> GUGCGACAAGAAGUUCAGGAAGGGAUUGAGGUGAAAGUCCUCCUCCCGAAUCGUUCAUGGGAGAGUCUAUCCAGACUUGCGUAGCGAGUAAUCGCUAGGUGAGAAGCUCUGGAGACAAUGUACCUGCCCUUCAAUUGGAGGUGCCAGGGCUAGGCUUUGUUCCUAUGGCUAGCGAAAGCGAAUACAGGUUAUUAGGCGUCGUGAAAACAAAACUCUUUCGACAUAAGGGAGAGGCUCGUAGAUGAGUUACCCUCCUUUUUAUGGGGUAACUGAACGAUCAAUAUCUACCGGCGUAGACUGUGAGCCUAAAGGAAACGAAUGAAAGUGUCCCUUCCUGGGAACUUGGUAAGCCCAAUAGACUCCCUCUGGGAAACCAGAGGAGGAGUAAGAGCAAUCUUACUUAUCGUCUAGUGGGUAAAAGACAUAAUAGGAAGCAAAUGCUUGGUUGUAACGAUCGAGAUAGAAUCUGUUGAUUUAAGCUGAAAGGCUGCAGACUUAUUAAAUGGGUGUUCUGCUGUAUGGCGUUCGCGCCUAAGCAGCAGAAUGCGUGAGCCGUGUGCGAUGAAAGUCGCAAGCACGGUUCUGAUGGGGGGAAAACGAGAGAUCGUCUACCUAUCCAACUCAA;> UGUUUAUUAAAAA

Group II introns are self-splicing ribozymes that catalyze two transesterification reactions to excise themselves from pre-messenger RNA. In the first step of splicing, the 2′-OH of a bulged adenosine residue is used as the nucleophile to attack the 5′ splice site. This is followed by a second step in which the free 3′-OH of the 5′ exon attacks the 3′ splice site to form ligated exons. In group II introns, the 3′ splice site is positioned in the core via domain VI and the IBS3-EBS3 interaction.

Here we report the 3.7 Å crystal structure of a eukaryotic group IIB intron from the brown algae Pylaiella littoralis (P.li.LSUI2) in the lariat-3′ exon form with an intact 3′ splice site docked into the catalytic core. The intact 3′ splice site is aligned in the active site adjacent to the two catalytic Mg2+ ions and the 3′-OH nucleophile of the 5′ exon. The presence of iridium hexammine promotes exon ligation, whereas its absence stalls splicing in crystallo prior to the second step. The scissile phosphate junction at the 3′ splice site is highly distorted and kinked as predicted by Chan et al. (2012). This distortion likely aids in presenting the correct scissile phosphate to the catalytic metal ions for cleavage in the second step in addition to applying strain on this bond to assist cleavage. γ-γ′ is not engaged in the observed pre-2s state, thus accounting for the 10 Å distance between the 3′ splice site and the catalytic metal ions M1 and M2. The γ nucleotide from J2/3 is flipped 180° away from the active site and therefore cannot pair with the 3′ terminal nucleotide (γ′) of the intron. The lack of this interaction accounts for the fact that the 3′ splice site is intact in this structure. In contrast to the post-catalytic structure, A586 of J5/6 has taken the place of U549 in the base triple below domain V and U549 is observed stacking underneath the nucleobase of the J2/3 residue G421.> MNESAGHNIKEDYFRVDMLLNKKGQVILYGPPGTGKTWIARKYVVEETNEKTPGNKWEFI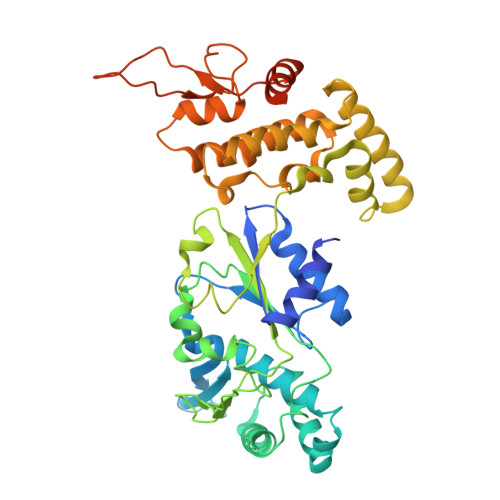TFHQSYSYEEFIEGFRPRTDNEEKIRYVVEDGIFKKIALRALVKGLFELEDATIGKDKIHRLYILLTKKEPLSPTEYEEYLRLKRYLWELVGGLPKDKLKNLTPKFYLIIDEINRGNISKIFGELITLLEKDKRLGGENQLIVRLPYSGEPFAVPPNLYIIGTMNTADRSIALLDVALRRRFAFIEVEPRPEFLEKENLKKIREKKLKTEDRKRLNEKLNELFSKLGNDNYFLKTLLEKINVRITVVKDRDHRIGHSYFLNVETVEDLHHVWYYEVLPLLMEYFYNDWETIKWVLNEKGKEHGNVFFEKLRLTGPNGEEAYQLKVLEGDAFIGALKRIISKNTPSQEGGATTNEENSPENTQSQTEGD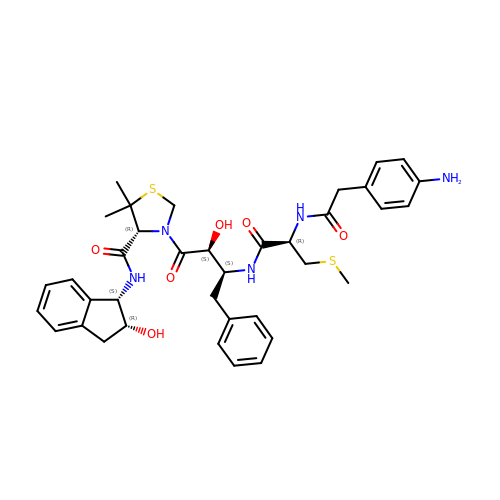(4R)-3-[(2S,3S)-3-[[(2R)-2-[2-(4-aminophenyl)ethanoylamino]-3-methylsulfanyl-propanoyl]amino]-2-oxidanyl-4-phenyl-butanoyl]-5,5-dimethyl-N-[(1S,2R)-2-oxidanyl-2,3-dihydro-1H-inden-1-yl]-1,3-thiazolidine-4-carboxamide | C37 H45 N5 O6 S2 | RYWMWBDZOSPVOM-ACUZRORGSA-N>[2x]GSDG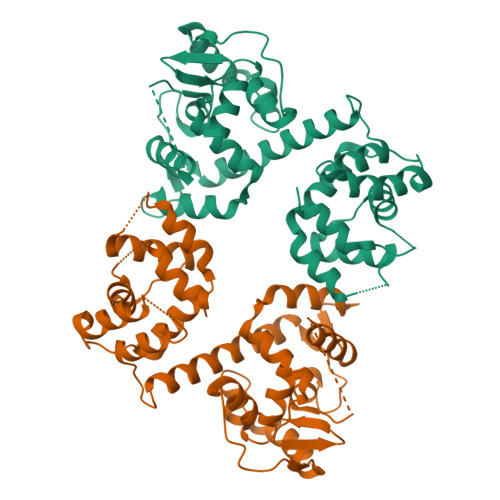SFTVSAQKNVEHGIIYIGKPSLRKQRFMQFSSLEHEGEYYMTPRDFLFSVMFEQMERKTSVKKLTKKDIEDTLSGIQTAGCGSTFFRDLGDKGLISYTEYLFLLTILTKPHSGFHVAFKMLDTDGNEMIEKREFFKLQKIISKQDDLMTVKTNETGYQEAIVKEPEINTTLQMRFFGKRGQRKLHYKEFRRFMENLQTEIQEMEFLQFSKGLSFMRKEDFAEWLLFFTNTENKDIYWKNVREKLSAGESISLDEFKSFCHFTTHLEDFAIAMQMFSLAHRPVRLAEFKRAVKVATGQELSNNILDTVFKIFDLDGDECLSHEEFLGVLKNRMHRG> MSNGDGLIRSLVDGDLEGFRQGFESFLDQCPSFLYHVSAGRFLPVFFFSMFSTAHDANILNANERVYFRFDNHGVNPRNGENRNTANLKVAVYRDGQQVVRCYSISDRPNSDGLRFSTRERNALVQEIRRQNPNLREEDLNFEQYKVCMHGKGKSQGEAIATVFEVIREKDRQGRDKFAKYSASEINLIRRLLGDHRLTIKEIEGRQLNQNQLRQLGRLVNFAQVAQGQQGIDNFMEMLASDRRQDVRDRIRREILPYITDIYNNYRQVLENNIENRNQRFEGHGFLLGFLANFSHRYTIGVDLDLSPRNSHVAFLVRHQVERENIPIVINLATRAPPYIALNRARSHAERLHVFSFIPIHTESRNTVCVGLNFNLNLDPFSVDTVGLQQDRFPLVQRLFECLENEGIRENIRDFLLHHLPAEIPRNAENYDRIFDCITGFAFGNSAFDRHPLELEEEDEAPITKYIFRHGDEGLRCLTMVFHAEGSDIVILHIRAHDAQQQGAINLQTLNVNGNDVHVWEVSCTLNNQLELDIDLPNDLGLYHDYQNNNANNFLA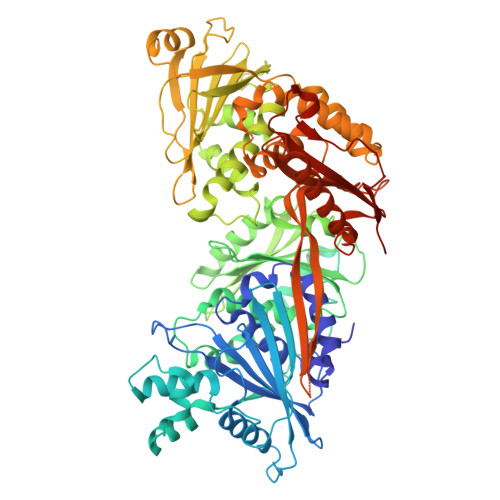GDLVQVPNTENVHNTLNQVVNDGWKNIAQHRGLFQEISGALMPLVDTINVNSEDKFRSILHGTFYASDNPYKVLAMYKVGQTYSLKRGQEEEGERVILTRITEQRLDLLLLRQPRENDLDTHPIGYVLRLANNAEEVGQQQNDARQEIGRLKKQHRGFIPITSGNEVVLFPIVFNRDAHEAGNLILFPEGIGREEHVHRLDRHVRLEHHHHHH> MTRGAWMCRQYDDGLKIWLAAPRENEKPFIDSERAQKWRLSLASLLFFTVLLSDHLWFCAEAKLTRTRDKEHHQQQQQQQQQQQQQQQQQQQQQQRQQQRQRQQQRQRQQEPSWPALLASMGESSPAAQAHRLLSASSSPTLPPSPG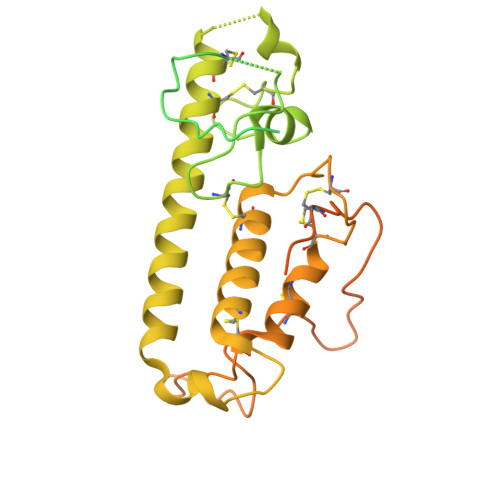GGGGSKGNRGKNNRSRALFLGNSAKPVWRLETCYPQGASSGQCFTVESADAVCARNWSRGAAAGEEQSSRGSRPTPLWNLSDFYLSFCNSYTLWELFSGLSSPSTLNCSLDVVLTEGGEMTTCRQCIEAYQDYDHHAQEKYEEFESVLHKYLQSDEYSVKSCPEDCKIVYKAWLCSQYFEVTQFNCRKTIPCKQYCLEVQTRCPFILPDNDEVIYGGLSSFICTGLYETFLTNDEPECCDIRSEEQTAPRPKGTVDRRDSCPRTSLTVSSATRLCPGRLKLCVLVLILLHTVLTASAAQNSTGLGLGGLPTLEDNSTRED>[8x]DDVTVVYQNGLPVISVRLPSRRERCQFTLKPISDSVGVFLRQLQEEDRGIDRVAIYSPDGVRVAASTGIDLLLLDDFKLVINDLTYHVRPPKRDLLSHENAATLNDVKTLVQQLYTTLCIEQHQLNKERELIERLEDLKEQLAPLEKVRIEISRKAEKRTTLVLWGGLAYMATQFGILARLTWWEYSWDIMEPVTY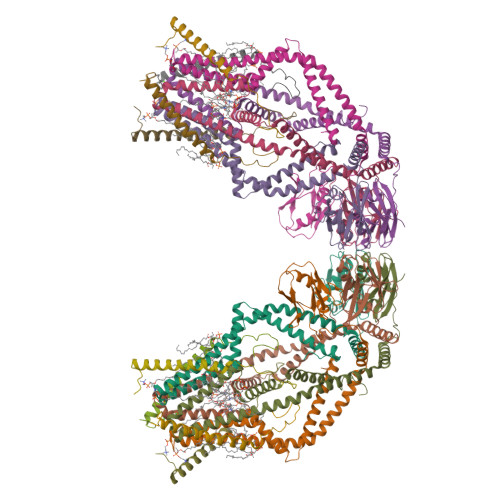FITYGSAMAMYAYFVMTRQEYVYPEARDRQYLLFFHKGAKKSRFDLEKYNQLKDAIAQAEMDLKRLRDPLQVHLPLRQIG;>[8x]VIVTRSGAILPKPVKMSFGLLRVFSIVIPFLYVGTLISKNFAALLEEHDIFVPE>MGSDKIHHHHHHENLYFQGAVVTVDGEVYGTYSLAKDQTIEIQDGNRLRIQNGQAKMEW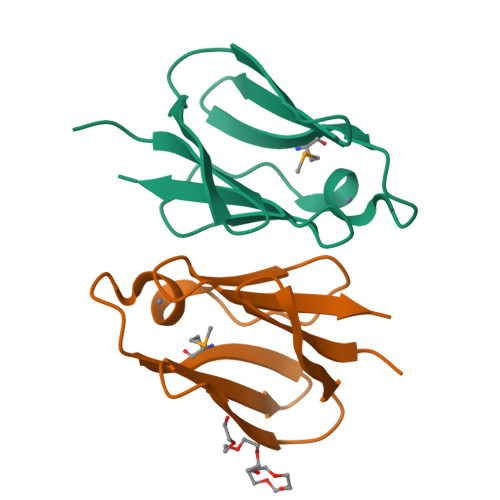ADCPDQLCVHQKAISRTGESIICLPNQVVVSVQGSKESELDGIVN[2x]>SGFVCNTCPEKWINFQRKCYYFGKGTKQWVHARYACDDMEGQLVSIHSPEEQDFLTKHASHTGSWIGLRNLDLKGEFIWVDGSHVDYSNWAPGEPTSRSQGEDCVMMRGSGRWNAAFCDRKLGAWVCD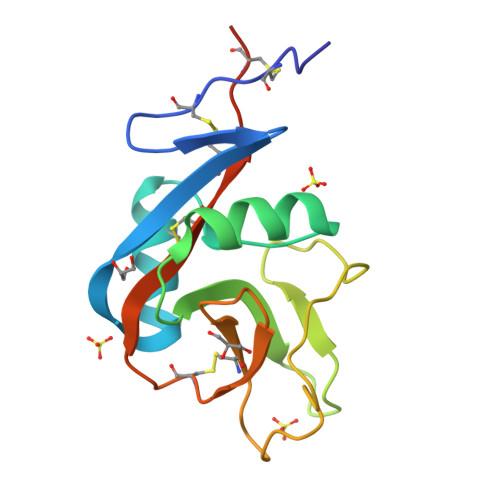RLATCTPPASEGSAE[7x]>[2x]VIEKVQHIQLLQKNVRAQLVDMKRLEVDIDIKIRSCRGSCSRALAREVDLKDYEDQQKQLEQVIAK;>HQLYIDETVNSNIPTNLRVLRSILENLRSKIQKLESDVSAQMEYCRTPCTVSCNIPVVSGKECEEIIRKGGETSEMYLIQPDSSVKPYRVYCDMNTENGGWTVIQNRQDGSVDFGRKWDPYKQGFGNVATNTDGKNYCGLPGEYWLGNDKISQLTRMGPTELLIEMEDWKGDKVKAHYGGFTVQNEANKYQISVNKYRGTAGNALMDGASQLMGENRTMTIHNGMFFSTYDRDNDGWLTSDPRKQCSKEAGGGWWYNRCHAANPNGRYYWGGQYTWDMAKHGTDDGVVWMNWKGSWYSMRKMSMKIRPFFPQQ[2x];>YE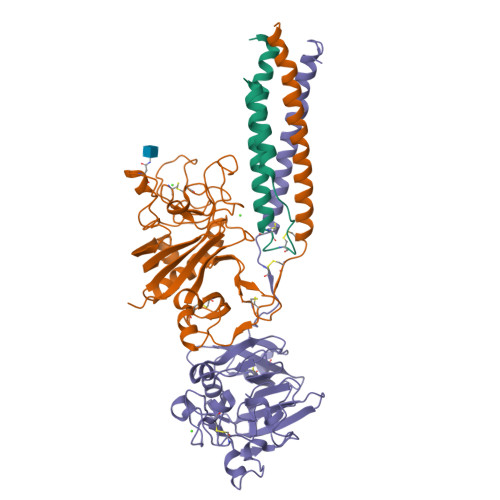ASILTHDSSIRYLQEIYNSNNQKIVNLKEKVAQLEAQCQEPCKDTVQIHDITGKDCQDIANKGAKQSGLYFIKPLKANQQFLVYCEIDGSGNGWTVFQKRLDGSVDFKKNWIQYKEGFGHLSPTGTTEFWLGNEKIHLISTQSAIPYALRVELEDWNGRTSTADYAMFKVGPEADKYRLTYAYFAGGDAGDAFDGFDFGDDPSDKFFTSHNGMQFSTWDNDNDKFEGNCAEQDGSGWWMNKCHAGHLNGVYYQGGTYSKASTPNGYDNGIIWATWKTRWYSMKKTTMKIIPFNRLTIGEGQQHHLGGAK[2x]2-sulfanylidene-1,7-dihydropyrrolo[2,3-d]pyrimidin-4-one 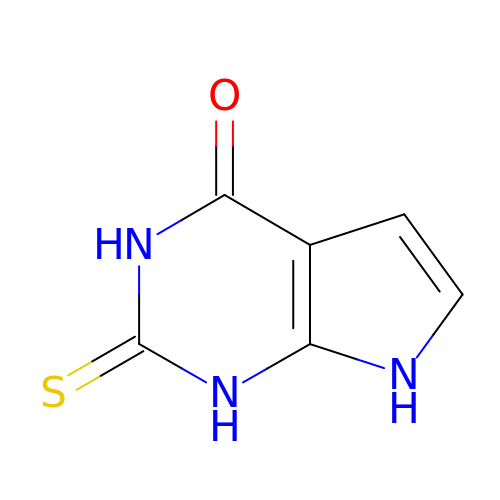| C6 H5 N3 O S | QCZHCRBHXAFBDJ-UHFFFAOYSA-N>MAHHHHHHMLKVTKAVFPVAGLGTRFLPATKASPKEMLPIVDKPLIQYAVEEAMAAGITEMIFVTGRSKRAIEDHFDKSYEIEAELQARGKDKLLELVRSIKPSHVDCFYVRQPEALGLGHAVLCAEKLVGDNPFAVILADDLLYGTPPVMAQMIEVFDHYHSSVIGVEEIPAQETKSYGIVDGKEWEDSIIKMSGIVEKPEPNVAPSNLGVVGRYVLKPRIFEHLRALKPGAGGELQLTDAIQSLLADEQVLAYKYHGTRFDCGSKLGYLKATVEFALRHP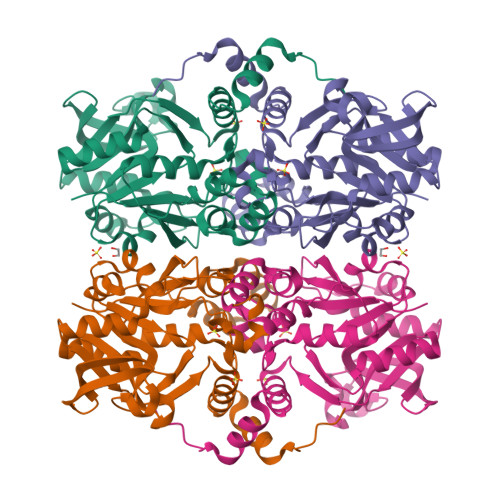EVAADFEEYLRTRSPVLEG[2x]While chemical methylation of an amide bond uses a strong base to generate the imidate, OphA, the precursor protein of the fungal peptide macrocycle omphalotin A, self-hypermethylates amides at pH 7 using S-adenosyl methionine (SAM) as cofactor. Omphalotin A derives from the C terminus of the OphA protein, and it is the OphA protein that methylates its own C terminus using S-adenosyl methionine (SAM). The structure of OphA reveals a complex catenane-like arrangement in which the peptide substrate is clamped with its amide nitrogen aligned for nucleophilic attack on the methyl group of SAM. Here, we report the structure of the peptide amide methyltransferase OphA including complexes with cofactor [SAM and S-adenosyl homocysteine (SAH)], cofactor analog, substrate, and product.

A second variant of OphA, truncated at Gly411 (OphAΔC6), containing the core peptide, is catalytically active with methylation of up to seven residues. Isolation and purification of OphAΔC6 after a short (2 hours) induction in E. coli yielded a less extensively methylated form (predominantly triply methylated). The location of the cofactor relative to the protein is identical in both the OphAΔC18 and OphAΔC6 complexes. The substrate peptide sits in the extended active-site tunnel with the amide nitrogen of Ile410 (we define the amide in this location as “i” hereafter) pointing toward the methyl group of SAM; the N(amide)-C(SAM)-S angle is 171°, close to the 180° required for an SN2 attack. The Ψ angle between residues i and i+1 is 0°. Consequently, the amide nitrogen atoms are arranged cis to each other, and the main chain twists 90°. Using structural superposition, we noted that placing (in silico) the larger SAM molecule into the SAH complex places the methyl group approximately 2.5 Å from substrate amide nitrogen. This clash is likely the reason why we have been unable to obtain fully occupied SAM complexes with active proteins. Although close contacts have been observed between SAM and its substrate in a number of structures, OphA appears to have the shortest distance.

>[2x]GTSTQTKAGSLTIVGTGIESIGQMTLQALSYIEAAAKVFYCVIDPATEAFILTKNKNCVDLYQYYDNGKSRLNTYTQMSELMVREVRKGLDVVGVFYGHPGVFVNPSHRALAIAKSEGYRARMLPGVSAEDCLFADLCIDPSNPGCLTYEASDFLIRDRPVSIHSHLVLFQVGCVGIADFNFTGFDNNKFGVLVDRLEQEYGAEHPVVHYIAAMMPHQDPVTDKYTVAQLREPEIAKRVGGVSTFYIPPKARKASNLDIIRRLELLPAGQVPDKKARIYPANQWEPDVPEVEPYRPSDQAAIAQLADHAPPEQYQPLATSKAMSDVMTKLALDPKALADYKADHRAFAQSVPDLTPQERAALELGDSWAIRCAMKNMPSSLLDAARESGEEASQNGFPWVIVVGVIGVIG>[2x]MVTAAISGTDEIRARAEQALTRCGVDLTAVKGDALTARTPLTGADLFGLRAQTPEDVDRAVEAAHTAFLTWRTTPAPVRGALVKRFGELLTEHKQDLADLVTIEAGKIRSEALGEVQEMIDICDFAVGLSRQLYGRTMPTERPGHRLMETWHPLGVVGVISAFNFPVAVWAWNAAVALVCGDTVVWKPS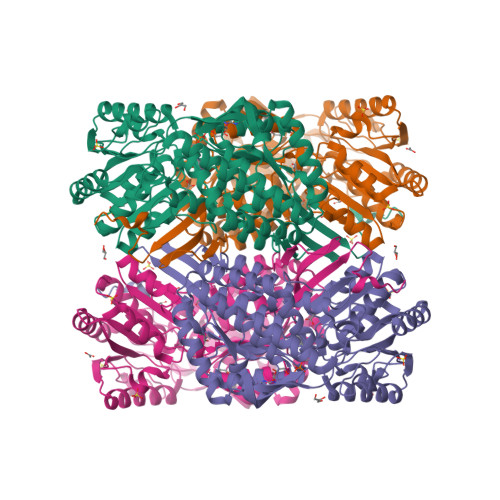ELTPLTALACAALLDLAIADAGAPKGLNQVVVGAADVGERLVDSPRVPLVSATGSTRMGRAVGPRVAARFGRTILELGGNNAAVVTPSADLDLTVNAAVFAAAGTAGQRCTTLRRLIVHEDIADTVVERLTAAFERLPIGDPFQDTTLVGPLVNEAAFGRMREAVERATAEGGTLCAGGERQFPDAAPGAYYVRPALVRMPAQTAVVREETFAPILYVLTYRDLDEAIRLNNEVPQGLSAGIFTADQSEAERFLAPDGADCGIANVNIGTSGAEIGGAFGGEKETGGGRESGSDAWRAYMRRATNTVNYSGRVTLAQGVDFSQ>[5x]MSKTVEDRAAQRAKGPATVLAIGTATPANVVYQTDYPDYYFRVTKSEHMTKLKNKFQRMCDRSTIKKRYMVLTEELLEKNLSLCTYMEPSLDARQDILVPEVPKLGKEAADEAIAEWGRPKSEITHLIFCTTCGVDMPGADYQLTKLLGLRSSVRRTMLYQQGCFGGGTVLRLAKDLAENNAGARVLVVCSEITTAVNFRGPSDTHLDLLVGLALFGDGAAAVIVGADPDPTLERPLFQIVSGAQTILPDSEGAINGHLREVGLTIRLLKDVPGLVSMNIEKCLMEAFAPMGIHDWNSIFWIAHPGGPTILDQVEAKLGLKEEKLKSTRAVLREYGNMSSACVLFILDEVRKRSMEEGKT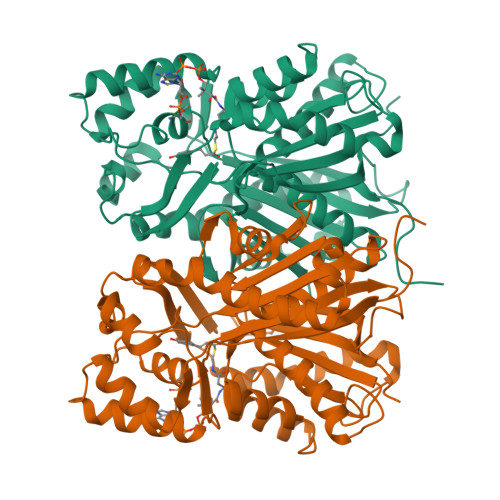TTGEGFDWGVLFGFGPGFTVETVVLHSMPIPKADEGR;> MSKTVEDRAAQRAKGPATVLAIGTATPANVVYQTDYPDYYFRVTKSEHMTKLKNKFQRMCDRSTIKKRYMVLTEELLEKNLSLCTYMEPSLDARQDILVPEVPKLGKEAADEAIAEWGRPKSEITHLIFCTTCGVDMPGADYQLTKLLGLRSSVRRTMLYQQGXFGGGTVLRLAKDLAENNAGARVLVVCSEITTAVNFRGPSDTHLDLLVGLALFGDGAAAVIVGADPDPTLERPLFQIVSGAQTILPDSEGAINGHLREVGLTIRLLKDVPGLVSMNIEKCLMEAFAPMGIHDWNSIFWIAHPGGPTILDQVEAKLGLKEEKLKSTRAVLREYGNMSSACVLFILDEVRKRSMEEGKTTTGEGFDWGVLFGFGPGFTVETVVLHSMPIPKADEGR> MGNLFGHKRWYEVRDKKDFKIKRKVKVKRNYDGNKYILNINENNNKEKIDNNKFIRKYINYKKNDNILKEFTRKFHAGNILFKLKGKEGIIRIENNDDFLETEEVVLYIEAYGKSEKLKALGITKKKIIDEAIRQGITKDDKKIEIKRQENEEEIEIDIRDEYTNKTLNDCSIILRIIENDELETKKSIYEIFKNINMSLYKIIEKIIENETEKVFENRYYEEHLREKLLKDDKIDVILTNFMEIREKIKSNLEILGFVKFYLNVGGDKKKSKNKKMLVEKILNINVDLTVEDIADFVIKELEFWNITKRIEKVKKVNNEFLEKRRNRTYIKSYVLLDKHEKFKIERENKKDKIVKFFVENIKNNSIKEKIEKILAEFKIDELIK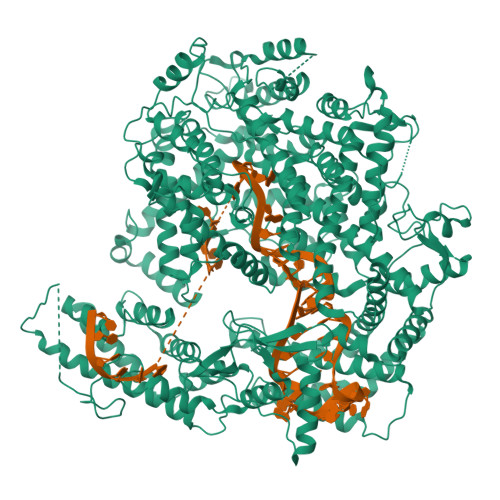KLEKELKKGNCDTEIFGIFKKHYKVNFDSKKFSKKSDEEKELYKIIYRYLKGRIEKILVNEQKVRLKKMEKIEIEKILNESILSEKILKRVKQYTLEHIMYLGKLRHNDIDMTTVNTDDFSRLHAKEELDLELITFFASTNMELNKIFSRENINNDENIDFFGGDREKNYVLDKKILNSKIKIIRDLDFIDNKNNITNNFIRKFTKIGTNERNRILHAISKERDLQGTQDDYNKVINIIQNLKISDEEVSKALNLDVVFKDKKNIITKINDIKISEENNNDIKYLPSFSKVLPEILNLYRNNPKNEPFDTIETEKIVLNALIYVNKELYKKLILEDDLEENESKNIFLQELKKTLGNIDEIDENIIENYYKNAQISASKGNNKAIKKYQKKVIECYIGYLRKNYEELFDFSDFKMNIQEIKKQIKDINDNKTYERITVKTSDKTIVINDDFEYIISIFALLNSNAVINKIRNRFFATSVWLNTSEYQNIIDILDEIMQLNTLRNECITENWNLNLEEFIQKMKEIEKDFDDFKIQTKKEIFNNYYEDIKNNILTEFKDDINGCDVLEKKLEKIVIFDDETKFEIDKKSNILQDEQRKLSNINKKDLKKKVDQYIKDKDQEIKSKILCRIIFNSDFLKKYKKEIDNLIEDMESENENKFQEIYYPKERKNELYIYKKNLFLNIGNPNFDKIYGLISNDIKMADAKFLFNIDGKNIRKNKISEIDAILKNLNDKLNGYSKEYKEKYIKKLKENDDFFAKNIQNKNYKSFEKDYNRVSEYKKIRDLVEFNYLNKIESYLIDINWKLAIQMARFERDMHYIVNGLRELGIIKLSGYNTGISRAYPKRNGSDGFYTTTAYYKFFDEESYKKFEKICYGFGIDLSENSEINKPENESIRNYISHFYIVRNPFADYSIAEQIDRVSNLLSYSTRYNNSTYASVFEVFKKDVNLDYDELKKKFKLIGNNDILERLMKPKKVSVLELESYNSDYIKNLIIELLTKIENTNDTLLEHHHHHH>GSHMSYNNIPAGKDAPNDIYVIIEIPANAAPIRYEIDKDSDALFVDRFMGTAMFYPANYGYVPNTLSEDGDPLDVLVVTPYPVAAGSVIRCRPVGKLNMEDDGGIDAKLIAVPHEKLSPLYKDVKEYTDLPQLLINQVEHFFSHYKDLEPGKWVKISGWEGADVAKAEVIKAIEAAK[8x]

However, because PPi is stable under normal conditions, inorganic pyrophosphatase (PPase) has evolved to specifically hydrolysis the molecule. Here, we solved four crystal structures of a family I type PPase from a strain of the pathogen Acinetobacter baumannii. The crystal structures of AbPPase showed that the enzyme has a typical Rossman fold domain that is highly conserved compared to other PPases. Family I PPases are hexamers formed by two stacks of trimers.

The space group of Structure 3 (K30R) is H32 with eight monomers in the asymmetry unit. In the enzyme assay, K30R lost the ability to hydrolyze PPi. Arg30 in the K30R adopts a different conformation compared to Lys30 in the WT enzyme. The side chain of Arg30 also affects the position of Arg44. Therefore, because of these differences, K30R could not be co-crystallized with PPi and also lost the ability to hydrolyze PPi (see the following section). The structure of K30R showed that the side chain of the Arg residue did not point in the same direction as the lysine residue in the WT enzyme. This suggests that Lys30 also plays a role in PPi binding. In contrast, K30R and K143R lost almost all the activity, demonstrating that Lys30 and Lys143 play key roles in AbPPase hydrolyzing activity. We also found that a highly conserved lysine residue (K30) in the AbPPase catalytic center is phosphorylated during PPi hydrolysis, and mutation of this lysine abolishes catalytic activity, suggesting that phosphorylated K30 is a catalytic intermediate.> MPSIAFSGISTKPGELEFHVPSVLSKHNRAGLLKSIDFPYSQRTIESSWNKLHYMESIRITPESRSVSVLLTDKESGDRVEMLAMVPLTTNKIIEISTATTDGTIILVTEEPHGFFAPGCFGKEVRNVISSYKSIFPHGTPPFILIHGSNGSVQVDPALFEYNDEYSVKIKYTAIRTEFKLFGKGDHGWMVTPEFPTISMLCQ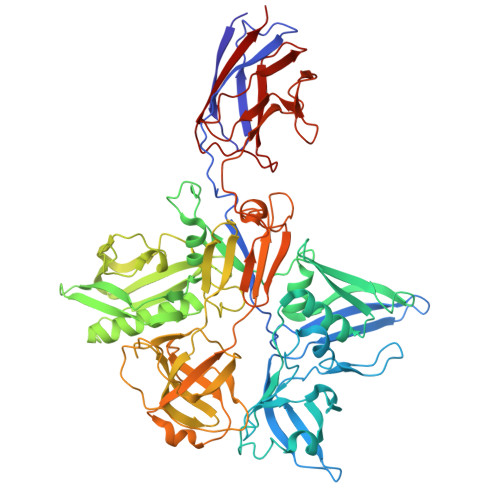VITNAMNSAIIFNHDDPAARTRMYPGTCSNTHVIESVSGDSLAKALLGYDGVYAGWEEITIPAGMYCYGELDLSKMIAAKMNRWHIDRESSIIFRGVSGYTWNVTLPSGNYGTPEKLAHCIQHMMNMTAKNRKNPYCVRFTLNEGSSHRGKFVFVAAEPFDLLFGDDESIDPSILGFEPVDHIGRNSYMSENDLGAPLMKPNCNVYDVDEIPGTHQIRIGRRTRLAVDGKIRGYSGGTLRLNTVNRTTGAPKCHGMNKGDVVTLTTVMPAPDGATGTKREGFTFRAKNKIMGVVVADENENPDASSLHVSVPSMSWTLGIGSYITIDSQAAPISVALFDPGKNQFFRDSIGASRLGFSNGVSTGQHGVVVSQCAVNLEPRTVDVSFIEGSMTSASTEMYNQNGKSLITQVPSDRSSGPVPQGMVRFNNALQQFKLEFTNPDGSPYHFNHASLSLLMEFDD> PVMLTPGSGQFLTTDDTQS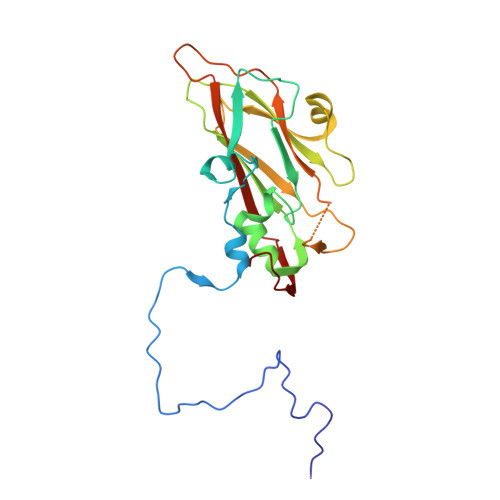PSAFPYFHPTKEIFIPGQVRNLIEMCQVDTLIPVNNTQENVRSVNMYTVDLRTQVDLAKEVFSIPVDIASQPLATTLIGELASYYTHWTGSLRFSFMFCGSASSTLKLLIAYTPPGVGKPKSRREAMLGTHLVWDVGLQSTASLVVPWVSASHFRFTTPDTYSSAGYITCWYQTNFVVPDSTPDNAKMVCMVSACKDFCLRLARDTNLHT> MNRFVIADSTLCIGCHTCEAACSETHRQHGLQSMPRLRVMLNEKESAPQLCHHCEDAPCAVVCPVNAITRVDGAVQLNESLCVSCKLCGIACPFGAIEFSGSRPLDIPANANTPKAPPAPPAPARVSTLLDWVPGIRAIAVKCDLCSFDEQGPACVRMCPTKALHLVDNTDIARVSKRKRELTFNTDFGDLTLFQQAQSGEAK;> MSAISLINSGVAWFVAAAVLAFLFSFQKALSGWIAGIGGAVGSLYTAAAGFTVLTGAVGVSGALSLVSYDVQISPLNAIWLITLGLCGLFVSLYNIDWHRHAQVKCNGLQINMLMAAAVCAVIASNLGMFVVMAEIMALCAVFLTSNSKEGKLWFALGRLGTLLLAIACWLLWQRYGTLDLRLLDMRMQQLPLGSDIWLLGVIGFGLLAGIIPLHGWVPQAHANASAPAAALFSTVVMKIGLLGILTLSLLGGNAPLWWGIALLVLGMITAFVGGLYALVEHNIQRLLAYHTLENIGIILLGLGAGVTGIALEQPALIALGLVGGLYHLLNHSLFKSVLFLGAGSVWFRTGHRDIEKLGGIGKKMPVISIAMLVGLMAMAALPPLNGFAGEWVIYQSFFKLSNSGAFVARLLGPLLAVGLAITGALAVMCMAKVYGVTFLGAPRTKEAENATCAPLLMSVSVVALAICCVIGGVAAPWLLPMLSAAVPLPLEPANTTVSQPMITLLLIACPLLPFIIMAICKGDRLPSRSRGAAWVCGYDHEKSMVITAHGFAMPVKQAFAPVLKLRKWLNPVSLVPGWQCEGSALLFRRMALVELAVLVVIIVSRGA;> MSVLYPLIQALVLFAVAPLLSGITRVARARLHNRRGPGVLQEYRDIIKLLGRQSVGPDASGWVFRLTPYVMVGVMLTIATALPVVTVGSPLPQLGDLITLLYLFAIARFFFAISGLDTGSPFTAIGASREAMLGVLVEPMLLLGLWVAAQVAGSTNISNITDTVYHWPLSQSIPLVLALCACAFATFIEMGKLPFDLAEAEQELQEGPLSEYSGSGFGVMKWGISLKQLVVLQMFVGVFIPWGQMETFTAGGLLLALVIAIVKLVVGVLVIALFENSMARLRLDITPRITWAGFGFAFLAFVSLLAA;> MSEEKLGQHYLAALNEAFPGVVLDHAWQTKDQLTVTVKVNYLPEVVEFLYYKQGGWLSVLFGNDERKLNGHYAVYYVLSMEKGHHHHHHHHHHGSTKCWITVRVEVDANKPEYPSVTPRVPAAVWGEREVRDMYGLIPVGLPDERRLVLPDDWPDELYPLRKDSMDYRQRPAPTTDAETYEFINELGDKKNNVVPIGPLHVTSDEPGHFRLFVDGENIIDADYRLFYVHRGMEKLAETRMGYNEVTFLSDRVCGICGFAHSTAYTTSVENAMGIQVPERAQMIRAILLEVERLHSHLLNLGLACHFTGFDSGFMQFFRVRETSMKMAEILTGARKTYGLNLIGGIRRDLLKDDMIQTRQLAQQMRREVQELVDVLLSTPNMEQRTVGIGRLDPEIARDFSNVGPMVRASGHARDTRADHPFVGYGLLPMEVHSEQGCDVISRLKVRINEVYTALNMIDYGLDNLPGGPLMVEGFTYIPHRFALGFAEAPRGDDIHWSMTGDNQKLYRWRCRAATYANWPTLRYMLRGNTVSDAPLIIGSLDPCYSCTDRMTVVDVRKKKSKVVPYKELERYSIERKNSPLK;> MFTFIKKVIKTGTATSSYPLEPIAVDKNFRGKPEQNPQQCIGCAACVNACPSNALTVETDLATGELAWEFNLGHCIFCGRCEEVCPTAAIKLSQEYELAVWKKEDFLQQSRFALCNCRVCNRPFAVQKEIDYAIALLKHNGDSRAENHRESFETCPECKRQKCLVPSDRIELTRHMKEAI;> MSNLLGPRDANGIPVPMTVDESIASMKASLLKKIKRSAYVYRVDCGGCNGCEIEIFATLSPLFDAERFGIKVVPSPRHADILLFTGAVTRAMRSPALRAWQSAPDPKICISYGACGN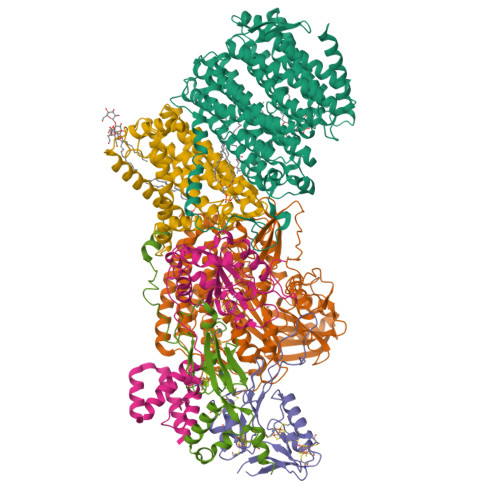SGGIFHDLYCVWGGTDKIVPVDVYIPGCPPTPAATLYGFAMALGLLEQKIHARGPGELDEQPAEILHGDMVQPLRVKVDREARRLAGYRYGRQIADDYLTQLGQGEEQVARWLEAENDPRLNEIVSHLNHVVEEARIR>[2x]AALQQDATPATREANQALYRKLPFADKTDFNNAHQGFIAPLPPAMLKGAQGNIIWDPAKYDFVKEGEKAPDTVNPSLWRQSQLLNIGGLFKVTDGVYQIRNLDLSNMTIIEGKTGITVIDPLLSAEPAKEALALYFAHRPKKPVVAVLFTHSHVDHYGGIRGVVDEADVKAGKVKIYAPAGFMEEAVSENIMAGTAMSRRASYMYGNLLKPDAKGQVGA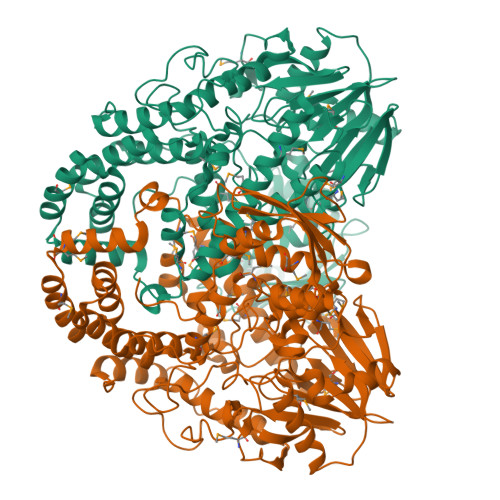GLGTTTSAGTVTLIPPTHYITHTGQQEVIDGLTYDFMMAPGSEAPSEMLWYVKEKKMIEAAEDVTHTLHNTYSLRGAKIRDPLAWSKYINAAIDRWGNEAEVIIAQHHWPTWGNDNIVKLMKGQRDMYRYINDQTLRMANLGMTRDEIAANFKLPDSLEKQWSSRGYYGSVSHDVKATYVFYLGWFDGNPATLDELPPEQAAKKFVEYMGGADAIMQKAKADYQQGNYRWVAQVTSKIVFADPDNQQARDLEADALEQLGYQAEAGTWRNFYLTGAQELRNGVQKLPTPNTASPDTVRAMTPEMFFDYLGVHINGEKAGAAKAVFNIDLGKDGGKYKLELENGVLNHTANAVADNADASISLSRDTLNKIILKQETLKQAEAQGKVKISGNGAKLDEMLSYMDTFAFWFNIVTP> MSQVWHNSNSQSNDVATSNDATGSNERNEKEPSLQGNKPGFVQQQQRITLPSLSALSTKEEDRRDSNGQQALTSHAAHILGYPPPHSNAMPSIATDSALKQPHEYHPRPKSSSSSPSINASLMNAGPAPLPTVGAASFSLSRFDNPLPIKAPVHTEEPKSYNGLQEEEKATQRPQDCKEVPAGVQPADAPDPSSNHADANDDNNNNENSHDEDADYRPLNVKDALSYLEQVKFQFSSRPDIYNLFLDIMKDFKSQAIDTPGVIERVSTLFRGYPILIQGFNTFLPQGYRIECSSNPDDPIRVTTPMGTTTVNNNISPSGRGTTDAQELGSFPESDGNGVQQPSNVPMVPSSVYQSEQNQDQQQSLPLLATSSGLPSIQQPEMPAHRQIPQSQSLVPQEDAKKNVDVEFSQAISYVNKIKTRFADQPDIYKHFLEILQTYQREQKPINEVYAQVTHLFQNAPDLLEDFKKFLPDSSASANQQVQHAQQHAQQQHEAQMHAQAQAQAQAQAQVEQQKQQQQFLYPASGYYGHPSNRGIPQQNLPPIGSFSPPTNGSTVHEAYQDQQHMQPPHFMPLPSIVQHGPNMVHQGIANENPPLSDLRTSLTEQYAPSSIQHQQQHPQSISPIANTQYGDIPVRPEIDLDPSIVPVVPEPTEPIENNISLNEEVTFFEKAKRYIGNKHLYTEFLKILNLYSQDILDLDDLVEKVDFYLGSNKELFTWFKNFVGYQEKTKCIENIVHEKHRLDLDLCEAFGPSYKRLPKSDTFMPCSGRDDMCWEVLNDEWVGHPVWASEDSGFIAHRKNQYEETLFKIEEERHEYDFYIESNLRTIQCLETIVNKIENMTENEKANFKLPPGLGHTSMTIYKKVIRKVYDKERGFEIIDALHEHPAVTAPVVLKRLKQKDEEWRRAQREWNKVWRELEQKVFFKSLDHLGLTFKQADKKLLTTKQLISEISSIKVDQTNKKIHWLTPKPKSQLDFDFPDKNIFYDILCLADTFITHTTAYSNPDKERLKDLLKYFISLFFSISFEKIEESLYSHKQNVSESSGSDDGSSIASRKRPYQQEMSLLDILHRSRYQKLKRSNDEDGKVPQLSEPPEEEPNTIEEEELIDEEAKNPWLTGNLVEEANSQGIIQNRSIFNLFANTNIYIFFRHWTTIYERLLEIKQMNERVTKEINTRSTVTFAKDLDLLSSQLSEMGLDFVGEDAYKQVLRLSRRLINGDLEHQWFEESLRQAYNNKAFKLYTIDKVTQSLVKHAHTLMTDAKTAEIMALFVKDRNASTTSAKDQIIYRLQVRSHMSNTENMFRIEFDKRTLHVSIQYIALDDLTLKEPKADEDKWKYYVTSYALPHPTEGIPHEKLKIPFLERLIEFGQDIDGTEVDEEFSPEGISVSTLKIKIQPITYQLHIENGSYDVFTRKATNKYPTIANDNTQKGMVSQKKELISKFLDCAVGLRNNLDEAQKLSMQKKWENLKDSIAKTSAGNQGIESETEKGKITKQEQSDNLDSSTASVLPASITTVPQDDNIETTGNTESSDKGAKIQ;> MVYEATPFDPITVKPSDKRRVAYFYDADVGNYAYGAGHPMKPHRIRMAHSLIMNYGLYKKMEIYRAKPATKQEMCQFHTDEYIDFLSRVTPDNLEMFKRESVKFNVGDDCPVFDGLYEYCSISGGGSMEGAARLNRGKCDVAVNYAGGLHHAKKSEASGFCYLNDIVLGIIELLRYHPRVLYIDIDVHHGDGVEEAFYTTDRVMTCSFHKYGEFFPGTGELRDIGVGAGKNYAVNVPLRDGIDDATYRSVFEPVIKKIMEWYQPSAVVLQCGGDSLSGDRLGCFNLSMEGHANCVNYVKSFGIPMMVVGGGGYTMRNVARTWCFETGLLNNVVLDKDLPYNEYYEYYGPDYKLSVRPSNMFNVNTPEYLDKVMTNIFANLENTKYAPSVQLNHTPRDAEDLGDVEEDSAEAKDTKGGSQYARDLHVEHDNEFY;>MVDLEQEFALGGRCLAFHGPLMYEAKILKIWDPSSKMYTSIPNDKPGGSSQATKEIKPQKLGEDESIPEEIINGKCFFIHYQGWKSSWDEWVGYDRIRAYNEENIAMKKRLANEAKEAKKSLLEQQKKKKLSTSLGGPSNGGKRKGDSRSNASISKSTSQSFLTSSVSGRKSGRSSANSLHPGSSLRSSSDQNGNDDRRRSSSLSPNMLHHIAGYPTPKISLQIPIKLKSVLVDDWEYVTKDKKICRLPADVTVEMVLNKYEHEVSQELESPGSQSQLSEYCAGLKLYFDKCLGNMLLYRLERLQYDELLKKSSKDQKPLVPIRIYGAIHLLRLISVLPELISSTTMDLQSCQLLIKQTEDFLVWLLMHVDEYFNDKDPNRSDDALYVNTSSQYEGVALGM[2x];>MDTSKKDTTRSPSHSNSSSPSSSSLSSSSSKEKKRPKRLSSQNVNYDLKRRKIITSEGIERSFKNEHSNLAVEDNIPEEEPKELLEKDSKGNIIKLNEPSTISEDSKVSVTGLPLNKGPSEKIKRESLWNYRKNLGGQSNNSEMTLVPSKRFTQVPKNFQDLNRNDLKTFLTENMTEESNIRSTIGWNGDIINRTRDREPESDRDNKKLSNIRTKIILSTNATYDSKSKLFGQNSIKSTSNASEKIFRDKNNSTIDFENEDFCSACNQSGSFLCCDTCPKSFHFLCLDPPIDPNNLPKGDWHCNECKFKIFINNSMATLKKIESNFIKQNNNVKIFAKLLFNIDSHNPKQFQLPNYIKETFPAVKTGSRGQYSDENDKIPLTDRQLFNTSYGQSITKLDSYNPDTHIDSNSGKFLICYKCNQTRLGSWSHPENSRLIMTCDYCQTPWHLDCVPRASFKNLGSKWKCPLHSPTKVYKKIHHCQEDNSVNYKVWKKQRLINKKNQLYYEPLQKIGYQNNGNIQIIPTTSHTDYDFNQDFKITQIDENSIKYDFFDKIYKSKMVQKRKLFQFQESLIDKLVSNGSQNGNSEDNMVKDIASLIYFQVSNNDKSSNNKSASKSNNLRKLWDLKELTNVVVPNELDSIQFNDFSSDEIKHLLYLKKIIESKPKEELLKFLNIENPENQSE[2x]

The Rpd3S complex plays a pivotal role in facilitating local histone deacetylation in the transcribed regions to suppress intragenic transcription initiation. Here, we present the cryo–electron microscopy structures of the budding yeast Rpd3S complex in both its apo and three nucleosome-bound states at atomic resolutions, revealing the exquisite architecture of Rpd3S to well accommodate a mononucleosome without linker DNA. The Rpd3S core, containing a Sin3 Lobe and two NB modules, is a rigid complex and provides three positive-charged anchors (Sin3_HCR and two Rco1_NIDs) to connect nucleosomal DNA. The Rpd3S core reveals a compact architecture composed of three modules: a Sin3 Lobe (Sin3 and Rpd3) and two modules involved in the nucleosome binding (named “NB1” and “NB2,” respectively).

We purified the endogenous Rpd3S complex from S. cerevisiae with all five known subunits by employing a C-terminal Flag-tag on Rco1. The EM maps allowed protein assignment and de novo atomic modeling covering six molecules for the Rpd3S complex, including Sin3, Rpd3, and two copies each of Rco1 (named as Rco1 and Rco1′) and Eaf3 (named as Eaf3 and Eaf3′). The extra EM map near the Sin3_HCR at a moderate local resolution may belong to the Ume1. The PAH1/2 of Sin3 and the NTD/PHD2 of Rco1 are unable to be modeled, likely due to their inherent flexibility. The Rpd3S core is almost identical in the apo- and three nucleosome-bound states, indicating that it is a rigid complex. The Sin3_HID/HCR and Rco1′_NTD wrap around the HDAC Rpd3. The Sin3_PAH3 catches an α helix of Rco1′_CTD. Two copies each of the Rco1_EID interacts with the Eaf3_MRG, forming the NB1 and NB2, respectively. The Rco1′_PHD1 in the NB2 is close to the active site of Rpd3, while the Rco1_PHD1 in the NB1 is far away. The central positioning of Rco1′_PHD2 within the complex serves to bridge the Sin3 Lobe and NB1/2, making a contribution to the stabilization of the Rpd3S core.>[2x]SMKDAPIINASKMNELMIQSSTILDRNENLVEKIENLENRTIVKLSDVPEHLINAFISTEDERFYSHKGVDPIGIAKSLIDTARGRIRGGSTIAQQLARNMYLSNERKIERKLKEAYLAIKITDSIKREGVLEAYLNRVFLGQHSYGVQSASQGYFSKDVKDLTIAESALLAAIVQSPTNYSLYKTIKPENVSDESAVIKDLNIGGQVYKAVYNPKVLDRQKYVLKKMYELKKITKEEYNNAVNEDVFS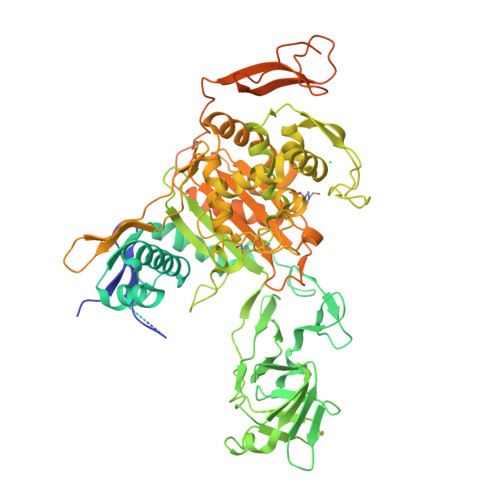AINPNKGFEREVSTYFTEYVKYQVAEKLMKKFNYTKEEAWDKIYNGGLTIHSTMDQNIQKNLEKLYADFANAMNAPRYGGPSFAAFKRDRASNITDEKGNIILYKKANLLDENNNVIIPKGEFSIDSDNSLKINSQRVSIYQNVLSMASFYTVNDQNNLVTHGIGNFQLPEQGVTVENEKSFKISASVFENYKDFYSVNENGNLVLNSKYFQVDEKGTVQPQSSSVVLDHKTGQLIAIIGGRETTGHPLNRAYRVPRQPGSTMKPLGVYIPALDNGYTAATAIEDAPHYNDKKELWPKNWYNGYRGLQTLRESLVQSINVNAVKTLEDIGIEKSKEYFKKFGLINEDNELDDTYVSRSESVDHNDENLSSMALGGMTRGMTNLKMTGAYAAIANDGRYNEPISFTKVVDSTGKTILEPEQKQRQVTSKENAFIMRDILKGVPDVMAHGAKHPTIEVSGKTGTTDDVQDSWFVGFTPYYTIGTWIGFDNQHIKLNNNNSMAATLWGKVNRIVLEGKEPKKFDGPSENIIRKYVSIRTGLLATEGTEKAIYEYFVKGTEPTKYEEIYYIAYKIDKRNGKLATDKTPEEFIEEKKFYIKPNVYKPEKTDYGPSDFINPPPTEESDIVDKPKEEEKPKTNTKPKTNDTSNKNDKDKDKDKDKDKDKNTEKDKNKNP> MKVAKDLVVSLAYQVRTEDGVLVDESPVSA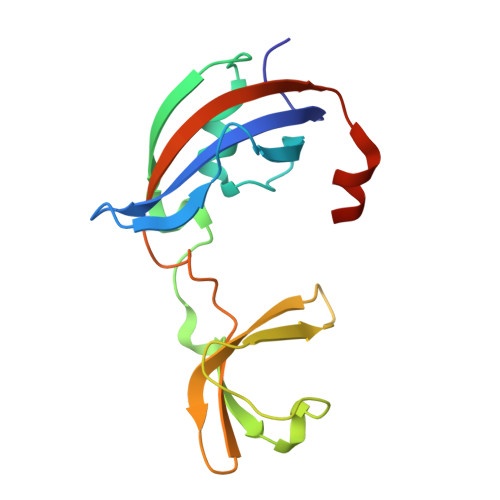PLDYLHGHGSLISGLETALEGHEVGDKFDVAVGANDAYGQYDENLVQRVPKDVFMGVDELQVGMRFLAETDQGPVPVEITAVEDDHVVVDGNHMLAGQNLKFNVEVVAIREATEEELAHGHVHG>GPGSMNVAISPGVTAGNSLPFVLFGGINV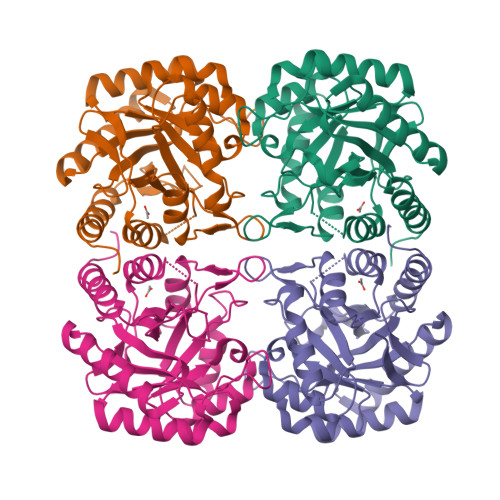LESLDFTLDVCGEYVAVTRKLGIPFVFKASFDKANRSSIHSYRGVGLDEGLKIFAEVKARFGVPVITDVHEAEQAAPVAEIADVLQVPAFLARQTDLVVAIAKAGKPVNVKKPQFMSPTQLKHVVSKCGEVGNDRVMLCERGSSFGYDNLVVDMLGFRQMAETTGGCPVIFDVTHSLQCRDPLGDASGGRRRQVLDLARAGIAVGIAGLFLEAHPDPDRARCDGPSALPLHQLEGLLSQMKAIDDLVKRMPALEIR[4x]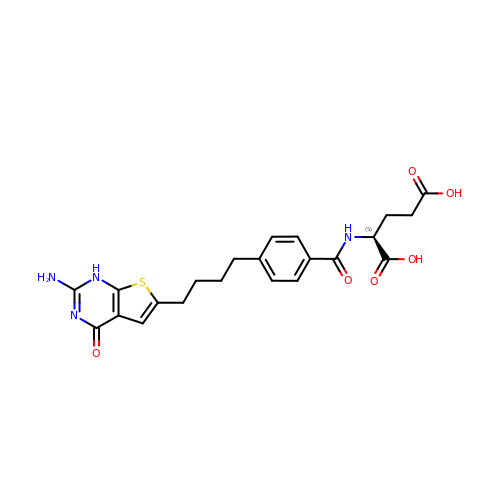N-{4-[4-(2-amino-4-oxo-1,4-dihydrothieno[2,3-d]pyrimidin-6-yl)butyl]benzoyl}-L-glutamic acid | C22 H24 N4 O6 S | KVBZUTNKUVNMNN-INIZCTEOSA-N>GMFVQSALHQLKVAVDTSIQMLDQYTEIDLKIAPIQSKRSLFEMYAHLSLICHADLLILNGSTEKELHTFYKEQTPETIAQMQKTMIQGYDLLSKTFLSYSNEQLAEMKTAYWGISYSRFEW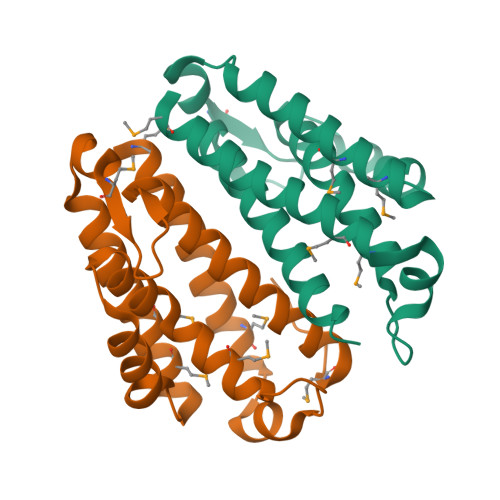LLEIVAHFYHHRGQIHILLCEHMKDPNIPLFQ[2x]> GSPIPHHDEKTWNVGSSNRNKAENLLRGKRDGTFLVRESSKQGCYACSVVVDGEVKHCVINKTATGYGFAEP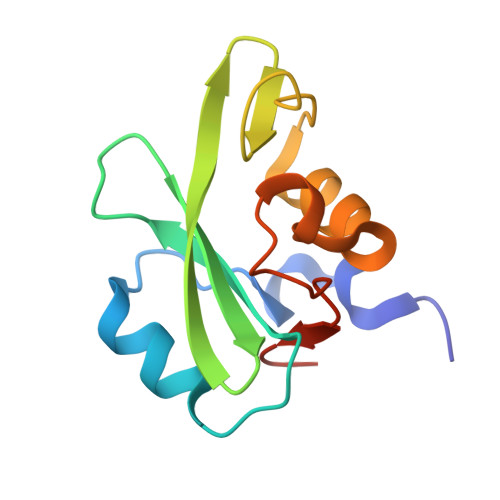YNLYSSLKELVLHYQHTSLVQHNDSLNVTLAYPVYAQQRR> GSMEDDAETKAKAEDLKMQGNKAMANKDYELAINKYTEAIKVLPTNAIYYANRAAAHSSLKEYDQAVKDAESAISIDPSYFRGYSRLGFAKYAQGKPEEALEAYKKVLDIEGDNATEAMKRDYESAKKKVEQSLNLEKTV

The yeast ortholog of SGTA, Sgt2, is best understood in the context of post-translational insertion of tail-anchored (TA) proteins into the ER membrane. Sgt2 captures TA substrates after they are released from the ribosome and passes them on to the Get3 ATPase, the central targeting complex, in a process mediated by the Get4/Get5 heterodimeric scaffolding complex. Sgt2 contains an N-terminal dimerization domain, followed by the conserved, central TPR domain and a glutamine rich region toward the C-terminus. Importantly for its role, Sgt2 associates with several heat-shock proteins such as Hsp104, Hsc82 (yeast ortholog of Hsp90), and Ssa1/Ssa2 (yeast orthologs of Hsp70), which can bind directly to its central TPR domain.

In this study, we report the first high resolution X-ray structure of the Sgt2_TPR at 1.55 Å and also in complex with the PTVEEVD peptide corresponding to the C-terminus of Ssa1, at 2.0 Å. The TPR domain of Sgt2 consists of three TPR repeats, comprising six almost identical α-helices and a C-terminal “capping” helix (α1 = A96-N115; α2 = Y118-V131; α3 = A136-L149; α4 = Y152-I165; α5 = F170-183Q; α6 = P186-E200; α7 = E206-L225) connected by short loops and arranged in a antiparallel fold homologous to that of SGTA_TPR. A structural overlay with the equivalent human domain is shown in Figure 1A (RMSD of 1.13 Å over 135 Cα). All residues were built into the electron density map except for the C-terminal Val229 and the solvent-exposed sidechains of Glu93 and Asp94. The final model also contains 90 water molecules and a single BO4 ion from the crystallization condition. It likely relates to the fact that the TPR domain helices suffer a subtle contraction to enclose the peptide in the TPR groove. The crystallographic structures we have obtained clearly show a slightly more compact conformation of the TPR where helices 1 and 7 are closer to each other in the complex structure than in the unbound TPR (See Figure S8 for a structural alignment).> L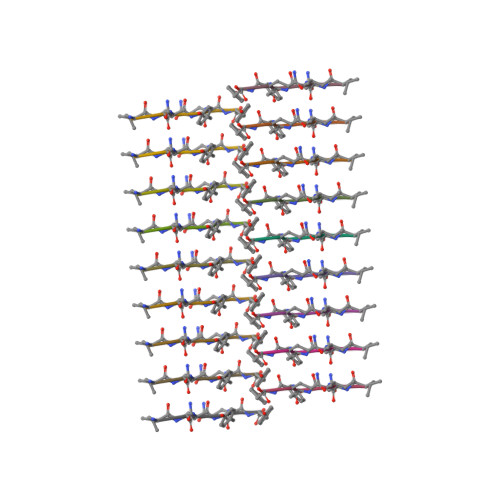NIYQY> MRFI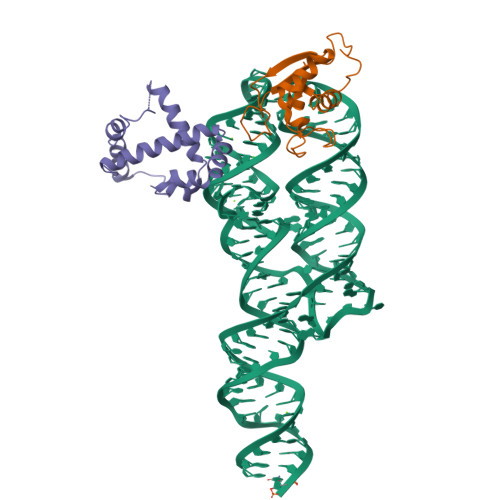CIYPAYLNNKKTIAEGRRIPISKAVENPTATEIQDVCSAVGLNVFLEKNKMYSREWNRDVQYRGRVRVQLKQEDGSLCLVQFPSRKSVMLYAAEMIPKLKTRTQ;> MRGSHHHHHHKHGQFTLRDMYEQFQNIMKMGPFSQILGMIPGFGTDFMSKGNEQESMARLKKLMTIMDSMNDQELDSTDGAKVFSKQPGRIQRVARGSGVSTRDVQELLTQYTKFAQMVKKMGGIKGLF Sirtuins are NAD+-dependent protein lysine deacylases that sense the cellular nutrient status, regulate energy metabolism and stress responses, and have been implicated in aging processes and aging-related diseases. Sirtuins feature differing substrate acyl selectivities. Here, we analyse modulation of Sirt6 and other isoforms by quercetin and its derivatives in activity and binding assays and through crystal structure analyses of modulator complexes of Sirt6 and Sirt2. Our results hence reveal sites and mechanisms for Sirtuin modulation by quercetin derivatives and provide helpful insights for Sirt6 modulator development.

To identify Sirt6’s quercetin binding site and interaction details, we determined a crystal structure of a Sirt6/ADP-ribose/quercetin complex at 1.84 Å resolution. Well-defined electron density for the quercetin ligand revealed the distal end of Sirt6’s extended acyl binding channel as binding site. The catechol moiety of quercetin (ring B) is buried in a protein pocket and its 4’-hydroxyl group forms a hydrogen bond to the Pro62 backbone oxygen, and the 4′- and 3'-hydroxyls form water-mediated interactions with the backbone of Ala53 and Ile61 and the side chain of Asp116. Asp116 normally forms a hydrogen bond to the NAM moiety of NAD+ bound in the so-called “C-site”, illustrating that catechol pocket and C-site partly overlap. The quercetin chromen-4-one system contributes to complex formation through hydrophobic contacts with funnel surface patches formed by Phe64/82/86 and Val70/115, and Met136/157. Comparison of the Sirt6/quercetin complex with a Sirt6 complex with the pyrrolo[1,2-a]quinoxaline-based activator UBCS039 shows that they share most of their binding sites. The catechol group of quercetin overlays well with the UBCS039 pyridine moiety and reproduces its key interaction to Pro6217. The chromen-4-one substitutes for the hydrophobic pyrrolo[1,2-a]quinoxalines of UBCS039-related compounds, which can vary between UBCS039 derivatives due to the non-directed nature of its interactions and the wide and hydrophobic architecture of the Sirt6 funnel. It thus appears that the buried catechol group of quercetin functions as an anchor in Sirt6 binding, while the chromen-4-one provides smaller and non-specific binding contributions and might be particularly amenable for modifications to increase compound affinity. Since quercetin occupies the distal end of the extended Sirt6 acyl channel it is compatible with binding of acetylated substrates but would overlap with longer substrate acylations such as myristoylations. Thus, quercetin stimulates the deacetylation activity of Sirt6 and inhibits Sirt6-dependent demyristoylations, as observed for UBCS039 and consistent with their binding to the remote end of the Sirt6 acyl channel.

>GIDPFTADKGKCGLPEIFDPPEELERKVWELARLVWQSSSVVFHTGAGISTASGIPDFRGPHGVWTMEERGLAPKFDTTFESARPTQTHMALVQLERVGLLRFLVSQNVDGLHVRSGFPRDKLAELHGNMFVEECAKCKTQYVRDTVVGTMGLKATGRLCTVAKARGLRACRGELRDTILDWEDSLPDRDLALADEASRNADLSITLGTSLQIRPSGNLPLATKRRGGRLVIVNLQPTKHDRHADLRIHGYVDEVMTRLMKHLGLEIPAWDGPRVLERALPPLPRPPTPKLEPKEESPTRIN[2x]N-(2,6-DIETHYLPHENYL)-1-METHYL-8-({4-[(1-METHYLPIPERIDIN-4-YL)CARBAMOYL]-2-(TRIFLUOROMETHOXY)PHENYL}AMINO)-4,5-DIHYDRO-1H-PYRAZOLO[4,3-H]QUINAZOLINE-3-CARBOXAMIDE | C35 H39 F3 N8 O3 | 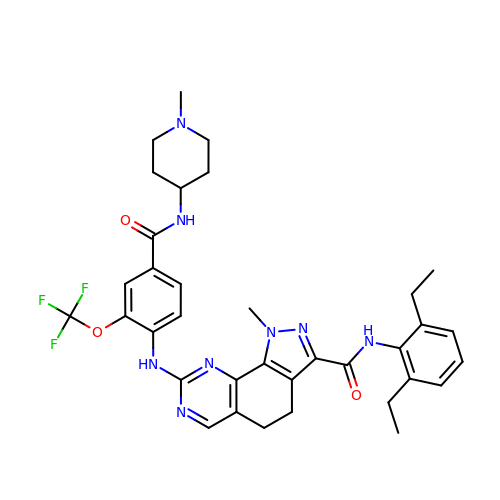JFOAJUGFHDCBJJ-UHFFFAOYSA-N> MEEPEEPADSGQSLVPV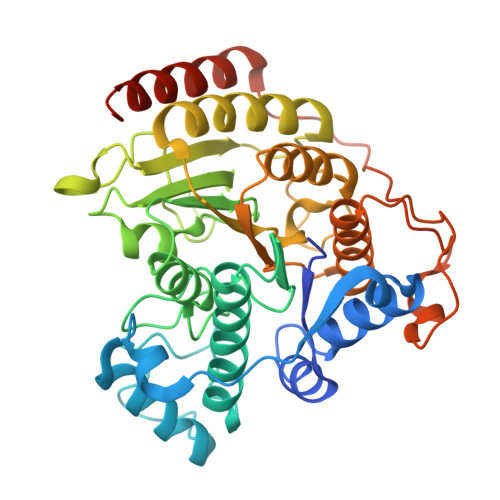YIYSPEYVSMCDSLAKIPKRASMVHSLIEAYALHKQMRIVKPKVASMEEMATFHTDAYLQHLQKVSQEGDDDHPDSIEYGLGYDCPATEGIFDYAAAIGGATITAAQCLIDGMCKVAINWSGGWHHAKKDEASGFCYLNDAVLGILRLRRKFERILYVDLDLHHGDGVEDAFSFTSKVMTVSLHKFSPGFFPGTGDVSDVGLGKGRYYSVNVPIQDGIQDEKYYQNCESVLKEVYQAFNPKAVVLQLGADTIAGDPMCSFNMTPVGIGKCLKYILQWQLATLILGGGGFNLANTARCWTYLTGVILGKTLSSEIPDHEFFTAYGPDYVLEITPSCRPDRNEPHRIQQILNYIKGNLKHVVIEGRGSHHHHHH> MVPISPIETVPVKLKPGMDGPKVKQWPLTEEKIKALVEICTEMEKEGKISKIGPENPYNTPVFAIKKKDSTKWRKLVDFRELNKRTQDFWEVQLGIPHPAGLKKKKSVTVLDVGDAYFSVPLDEDFR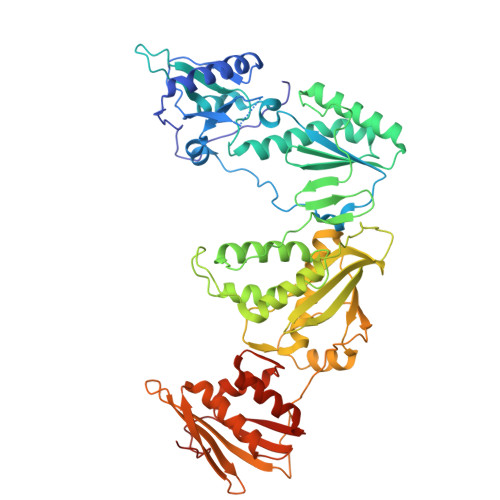KYTAFTIPSINNETPGIRYQYNVLPQGWKGSPAIFQSSMTKILEPFAAQNPDIVICQYMDDLYVGSDLEIGQHRTKIEELRQHLLRWGLTTPDKKHQKEPPFLWMGYELHPDKWTVQPIVLPEKDSWTVNDIQKLVGKLNWASQIYPGIKVRQLSKLLRGTKALTEVIPLTEEAELELAENREILKEPVHGVYYDPSKDLIAEIQKQGQGQWTYQIYQEPFKNLKTGKYARMRGAHTNDVKQLTEAVQKITTESIVIWGKTPKFKLPIQKETWETWWTEYWQATWIPEWEFVNTPPLVKLWYQLEKEPIVGAETFYVDGAANRETKLGKAGYVTNKGRQKVVPLTNTTNQKTELQAIYLALQDSGLEVNIVTDSQYALGIIQAQPDKSESELVNQIIEQLIKKEKVYLAWVPAHKGIGGNEQVDKLVSAG> TSNEVAQFLSKENQVIVRMRGLPFTATAEEVVAFFGQHCPITGGKEGILFVTYPDGRPTGDAFVLFACEEYAQNALRKHKDLLGKRYIELFRSTAAEVQQVLNRFSSAPLIPLPTPPII

The full-length ESRP1 is predicted to contain an RNase H-like domain and three quasi-RNA-recognition motifs (qRRMs) similar to those in hnRNP F. ESRP1 has been shown to control alternative splicing of multiple genes during EMT, many of which contribute to alterations in the actin cytoskeleton and cell motility. We found that the formation of this circRNA is dependent on the splicing regulator ESRP1, which promotes circDOCK1(2–27) formation by inhibiting splicing of exon 1 to exon 2, thereby holding the intron 1 acceptor site unspliced and available while Pol II completes its 157 kb journey from exon 2 to exon 27. We found by HITS-CLIP analysis that ESRP1 binds to a GU-rich motif in a tandem repeat region in intron 1.

Crystals that diffracted to 1.65A with space group P3121 were obtained for the ESRP1 qRRM2 domain complexed to a 12-mer RNA with sequence UGGUGGUGGUGG. The qRRM2 comprises four β-stands flanked by two alpha-helices at each side of the β-sheet. These helixes cover the beta-sheet region, making the qRRM domain different from canonical RRM domains, in which the RNA-binding region is located at the beta-sheet region, whereas the qRRM2 of ESRP1 binds to the RNA substrate through loop regions. The structure shows contacts with just three nucleotides of the RNA, with the sequence GGU binding within a double clamp arrangement. The three nucleotides are accommodated into a positively charged region, with two loop regions important for nucleotide binding, one of which is between β1 and α2 (Loop12 in Figure 5D) and another one between α3 and β4 (Loop34). The three nucleotide bases face down to Loop12 and Loop34, and the phosphate groups of the RNA are distal from the protein backbone, enhancing the sequence-specific RNA recognition by qRRM2. A close view of the interactions reveals that the two guanine residues are inserted into two clamps separated by Arg397 and form a π–π stacking like a sandwich. For G1 recognition, besides the stacking interactions from Arg397 and Phe335, the base of G1 is also specifically recognized through a number of hydrogen bonds. G2 is clamped by the side chain of Arg397 and Tyr398. Mutating each of the three important residues Phe335, Arg397 and Tyr398 to alanine resulted in the loss of RNA binding ability, and the R331A and E400A mutants showed dramatically decreased RNA binding affinity, consistent with the observations in the complex structure.> NRIITEYILIDANNYHFKSWIECFPDCKVNLKLLLFRPEWFDF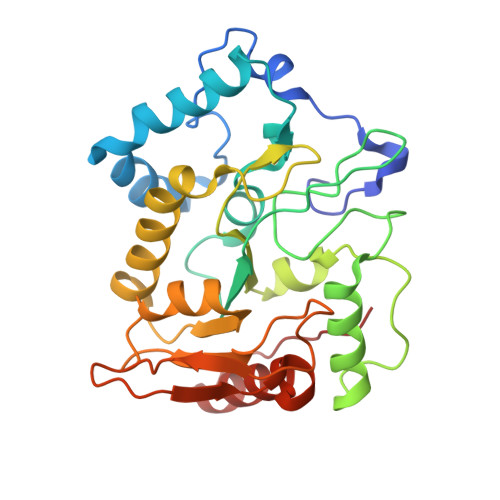FKYVESKTYFPQLESKLSSYLEKRQRIVPYPELLFNTMNVLPPGKIKVVILGQDPYPGSCISGVPYAMGCSFSVPLNCPVPKSLANIYTNLIKFNHMRKAPKHGCLASWILQGTFMINSAFTTVLNESGVHARTWESFTADLIDYLTDNYDDLIFVAWGAHAHKLCQRVDPKKHYIITSSHPSPFSVSNTMTSMSYGPNPKKVTYPSFNSVDHFGKINEHLKSRNKKPIFWDL> MATILLSAAGAAIGGGFGGTVLGLSGAVIGRAVGATLGRVIDQRLLGSGSQSVETG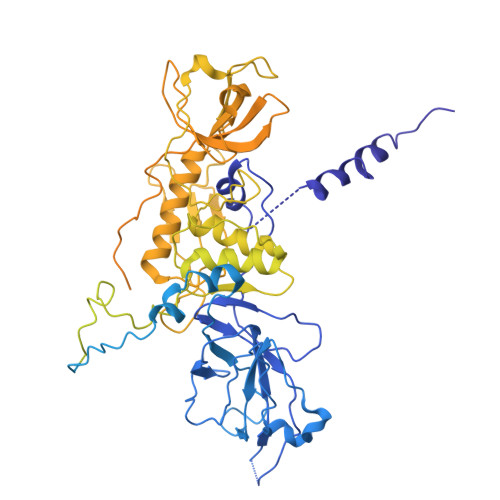RVDRLRLSSASEGEAVGRLWGRMRVAGQVIWATRFFESASVEKSGKGVPRATVTSYSYSLSLALALCEGEILRVGRVWADGSEIEVSGLNMRVYRGGEDQLPDPKIAAVEGAEAAPAYRGIAYVVLEDLQLAPFGNRVPQFTFEVVRAAQGALAEAEPDLTRGLRAVALIPGTGEYALATTPVYLATGSGVTATQGVANQNAPGGQTDLVAALERLDEELPNCGAVSLVVSWFGDDLRCGACDVKPKVASVAEEGANMPWRVAGLERAGAEEVPRLSGQSVYGGTPADAAVIEAIAALRAAGKAVTFYPFILMAQLAGNGLPDPWNPGSAQPALPWRGRITLSVAPGRAGSPDGTAAAEAQVAGFFGAASPGDSAIAGGEVVYSGPEEWSMRRFILHYAHLCQLAGGVDAFCIGTEMVALTQIRGPSNSFPAVAAFRQLAGEVKAILGPGCKIGYAADWSEYWGYAPGNGERFFHLDPLWADENIDFIGIDNYLPLSDWRDGADHADAGWGSIHALDYLRSNIEGGEYYDWFYAAPEHRAAQIRTPITDGDHDEPWIWRAKDLRNWWLNDHHERVGGLRSEVATAWVPQSKPIWFTEMGCAAIDKGTNQPNKFLDPKSSESGLPHHSDGRRDELIQMQYLRAMTGYWGEAARNPVSAVYGGPMLDMSRAHVWAWDARPWPQFPLNTALWSDGENYARGHWISGRAVAQPLASVVAEICGAAGITEIDVSGLYGLVRGYTMTGDQTGRAGLQALMLAYGFEALERDGQLVFRMRDGRVAADLAAADLALGEGEAVVETVRAAEAEIAGRVRLAYVEAEGDFEVKAVEAVFPDAAAGAAAGSELSLALTRAQAQGIVGRWLAEARVARDTARFALPPSRGHLGTGDVVRLDLPEGKRRYRIDRVEQAGLIQVEAVRVEPGIYAPADEVEDPASLRPFAAPVPVTAVFLDLPLMKGDEDPVAPHLAVTATPWPGTVAVWSSDEDAGYALNASLGTRAVIGQTLTPLFRARPGVWDRGAALRVRLASGALDSATAAKVLNGANAMAIGDGSSENWEVFQFAEAALVEGKIWDISLRLRGQLGTDALMPEVWPEGSVVVALNGAPEQILLPSAARGLARHYRIGAAVRSYDDPSFVHRIEAFAGAGLRPFSPCHLRAEPGASGWAFRWVRRTRIDGDSWQGYEVPLGETAELYLVRVLEGTAVKREVTVGEASWSYPAALQAADGIAGAFTLEVAQVSDVYGPGLAARITVGA4-FLUOROBENZYLAMINE 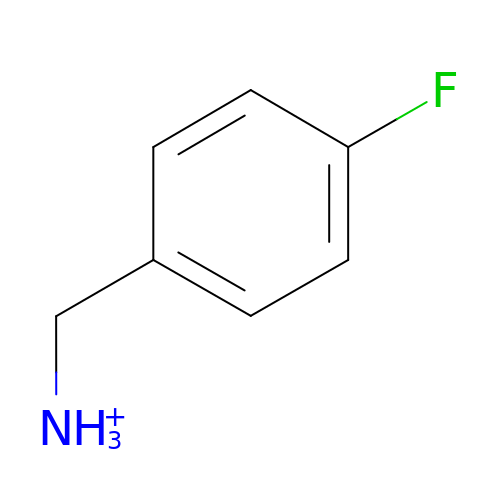| C7 H9 F N | IIFVWLUQBAIPMJ-UHFFFAOYSA-O> GAMVMRLGDAAELCYNLTSSYLQIAAESDSIIAQTQRAINTTKSILINETFPKWSPLNGEISFSYNGGKDCQVLLLLYLSCLWEYYIVKLSQSQFDGKFHRFPLTKLPTVFIDHDDTFKTLENFIEETSLRYSLSLYESDRDKCETMAEAFETFLQVFPETKAIVI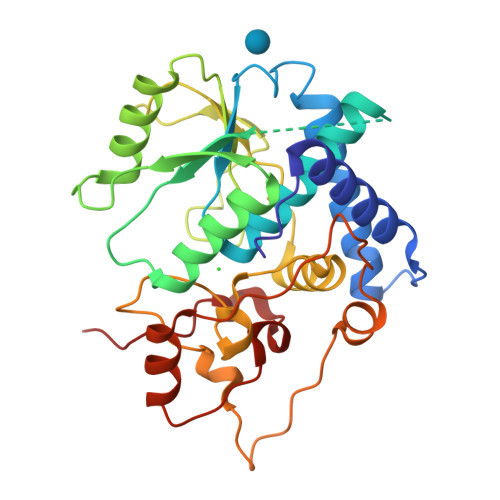GIRHTDPFGEHLKPIQKTDANWPDFYRLQPLLHWNLANIWSFLLYSNEPICELYRYGFTSLGNVEETLPNPHLRKDKNSTPLKLNFEWEIENRYKHNEVTKAEPIPIADEDLVKIENLHEDYYPGWYLVDDKLERAGRIKKK> IVGGTNSSWGEWPWQVSLQVKLTAQRHLCGGSLIGHQWVLTAAHCFDGLPLQDVWRIYSGILNLSDITKDTPFSQIKEIIIHQNYKVSEGNHDIALIKLQAPLNYTEFQKPISLPSKGDTSTIYTNCWVTGWGFSKEKGEIQN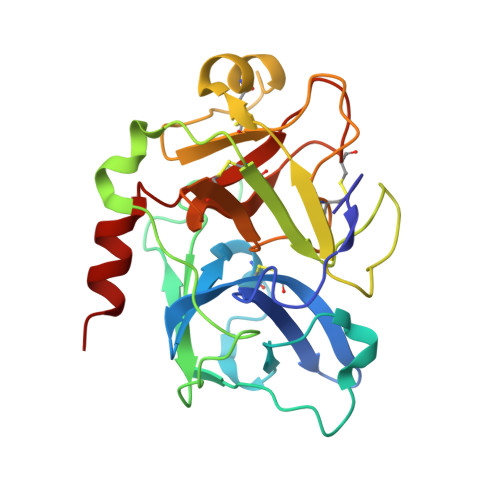ILQKVNIPLVTNEECQKRYQDYKITQRMVCAGYKEGGKDACKGDSGGPLVCKHNGMWRLVGITSWGEGCARREQPGVYTKVAEYMDWILEKTQS>[12x]GPLGSPEFRYFVA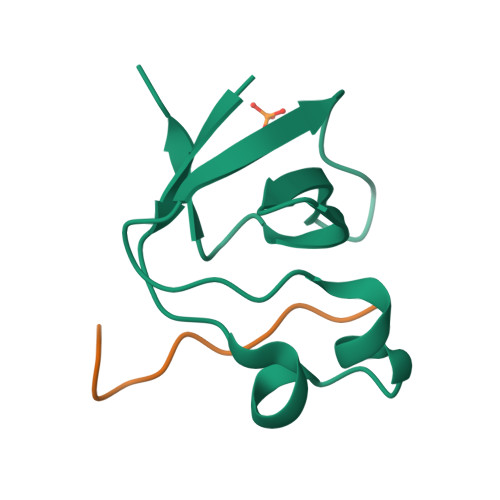MFDYDPSTMSPNPDGCDEELPFQEGDTIKVFGDKDADGFYWGELRGRRGYVPHNMVSEVE;>XTRRRRKLPEIPKNKKX[12x]N-OMEGA-PROPYL-L-ARGININE | C9 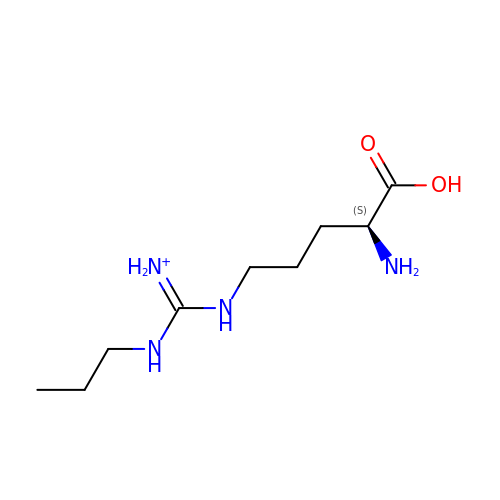H21 N4 O2 | AOMXURITGZJPKB-ZETCQYMHSA-O beta-cyclocitral | C10 H16 O | 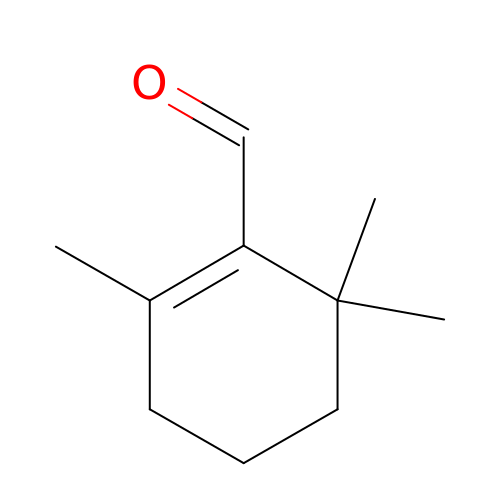MOQGCGNUWBPGTQ-UHFFFAOYSA-N>MKKLFLVFWWHMHQPLYREPYTGEYLLPWTFFHAVKDYYDMPAYLKDFEIKLNFNLTPVLIDQIQEYAQGKAKDVFLEAIRKDPDDLEKEEVEKLIEFTKLNYEKPIYRFERIRELMNKEKLNREELLDLQTLNLLAWCGRTLRKDLKDLLNKGRNYTQEEKEYVLNKYFEIIKKTLSIYREIKEEGKGSVSTSPYYHPLIPILLNPNCVYETTPNVKIPDFAVSFREDASKHVELAKEKYFEIFGEHPVYMWPPEASVSNEALELYYEKGINMLATDEVILKNSVERASPYLRYYFRELISVFFRDKTLSDLIGFSYHAWNAEDAVRDFIGRLKKIHESVDFQPVVFVVLDGENCWEYYEENGIPFLEKLYSTLEKEEWIETLTLEEAMRKEDVKTEVIESVKAGTWFDGNFLKWIGNKEKNEYWKILIEAKKKAKNDYILVAEG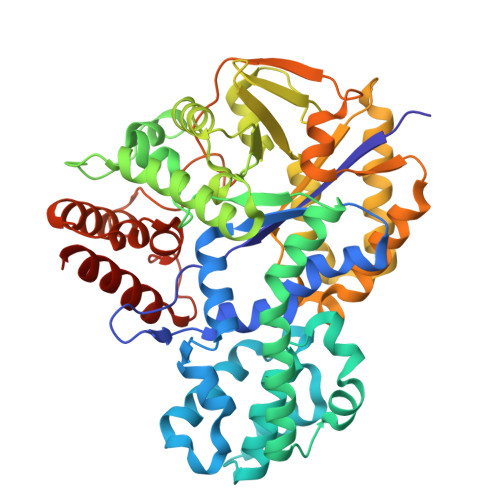SDWFWWQGEEKAPFVEVFDKLFRSFVRRAQELEHHHHH[4x]> MGSSHHHHHHSSGLVPRGSTQTVHEFAKELDATNISIDKVVGAGEFGEVCSGRLKLPSKKEISVAIKTLKVGYTEKQRRDFLGEASIMGQFDHPNIIRLEGVVTKSKPVMIVTEYMENGSLDSFL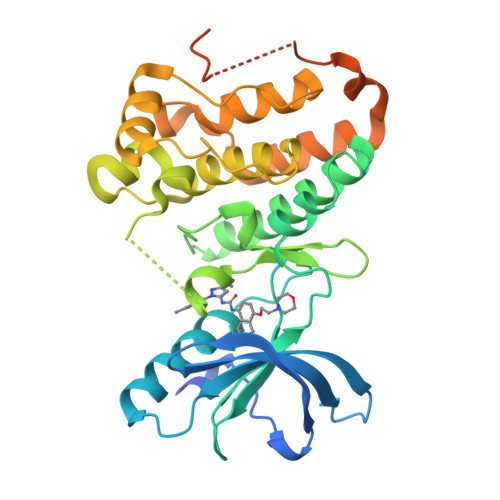RKHDAQFTVIQLVGMLRGIASGMKYLSDMGYVHRDLAARNILINSNLVCKVSDFGLSRVLEDDPEAAYTTRGGKIPIRWTSPEAIAYRKFTSASDVWSYGIVLWEVMSYGERPYWEMSNQDVIKAVDEGYRLPPPMDCPAALYQLMLDCWQKDRNNRPKFEQIVSILDKLIRNPGSLKIITSAAARPSNLLLDQSNVDITTFRTTGDWLNGVWTAHCKEIFTGVEYSSCDTIAKIS In the nucleoplasm, however, hMTR4 binds the RBM7 and ZCCHC8 proteins, forming the metazoan-specific nuclear exosome targeting (NEXT) complex27. NEXT promotes the exosomal degradation of non-coding promoter-upstream transcripts, enhancer RNAs28 and 3′-extended products of histone- and small nuclear RNA transcription. We conclude that ZCCHC8 is a scaffolding subunit that bridges the interaction between RBM7 and hMTR4. In this work, we have shown that RBM7RRM binds a proline-rich segment of ZCCHC8 at the back helical surface and is able to concomitantly bind RNA.

To obtain experimental phases, we co-crystallized the complex in the presence of heavy-atom compounds. Co-crystallization with Samarium chloride yielded a different crystal form diffracting to 2.0 Å resolution and containing a single copy of the complex in the asymmetric unit. The structure was solved by single anomalous dispersion at the Samarium edge and refined to 2.0 Å resolution with Rfree of 22.6%, R-factor of 20.2% and good stereochemistry. As the two structures are very similar, we focused on the highest-resolution atomic model, which includes residues 286–324 of ZCCH8 and residues 7–86 of RBM7. Side-chain electron density was well resolved throughout the RBM7RRM–ZCCHC8Pro interface. In the complex, RBM7RRM exposes the front β-sheet surface to solvent and engages the helical back surface in binding ZCCHC8Pro with conserved interactions. Overall, ZCCHC8Pro adopts an unusual elliptical conformation when bound to RBM7. The RBM7RRM–ZCCHC8Pro interaction is dominated by conserved hydrophobic contacts that can be grouped into two adjacent patches. The first interaction hotspot (patch 1) is in the lower half of the RRM domain: ZCCHC8Pro helix αA together with the preceding and following loops insert a set of apolar residues into a shallow hydrophobic pocket formed between the α1 and β4add elements of RBM7RRM.

> GPDSMGAAAAEADRTLFVGNLETKVTEELLFELFHQAGPVIKVKIPKDKDGKPKQFAFVNFKHEVSVPYAMNLLNGIKLYGRPIKIQFRS;> GPDSMRFKPGVISEELQDALGVTDKSLPPFIYRMRQLGYPPGWLK>[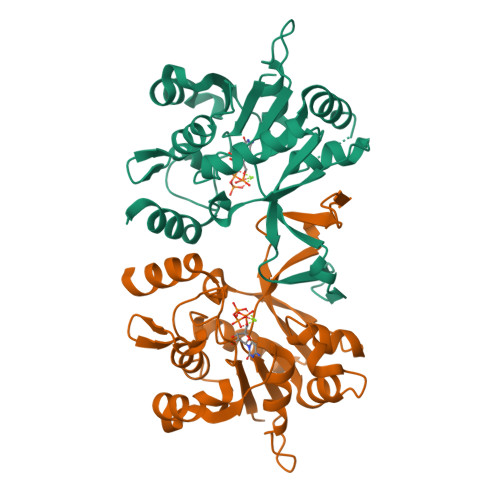2x]VVREAGEVVAIVPAAGSGERLAVGVPKAFYQLDGQTLIERAVDGLLDSGVVDTVVVAVPADRTDEARQILGHRAMIVAGGSNRTDTVNLALTVLSGTAEPEFVLVHDAARALTPPALVARVVEALRDGYAAVVPVLPLSDTIKAVDANGVVLGTPERAGLRAVQTPQGFTTDLLLRSYQRGSLDLPAAEYTDDASLVEHIGGQVQVVDGDPLAFKITTKLDLLLAQAIVRG(3P,5M)-3-{3-[(3,5-dichloropyridin-2-yl)oxy]phenyl}-5-(1H-tetrazol-5-yl)-2,1-benzoxazole | 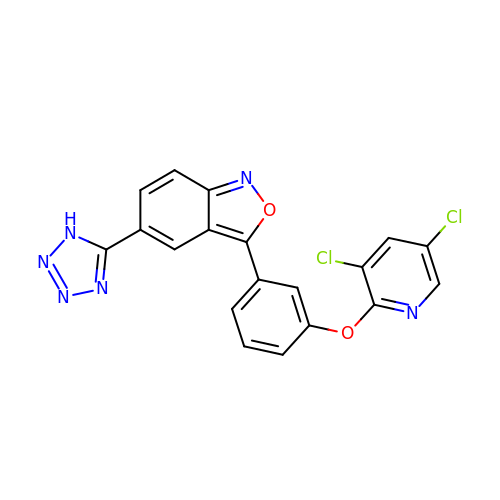C19 H10 Cl2 N6 O2 | HUCBOYYRZGDAFL-UHFFFAOYSA-N>[6x]MNLTELKNTPVSELITLGENMGLENLARMRKQDIIFAILKQHAKSGEDIFGDGVLEILQDGFGFLRSADSSYLAGPDDIYVSPSQIRRFNLRTGDTISGKIRPPKEGERYFALLKVNEVNFDKPENARNKILFENLTPLHANSRLRMERGNGSTEDLTARVLDLASPIGRGQRGLIVAPPKAGKTMLLQNIAQSIAYNHPDCVLMVLLIDERPEEVTEMQRLVKGEVVASTFDEPASRHVQVAEMVIEKAKRLVEHKKDVIILLDSITRLARAYNTVVPASGKVLTGGVDANALHRPKRFFGA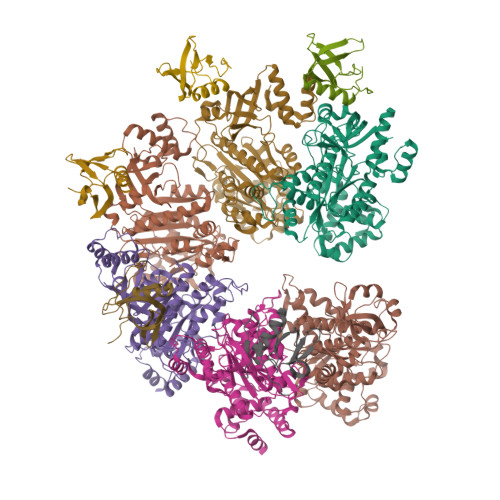ARNVEEGGSLTIIATALIDTGSKMDEVIYEEFKGTGNMELHLSRKIAEKRVFPAIDYNRSGTRKEELLTTQEELQKMWILRKIIHPMGEIDAMEFLINKLAMTKTNDDFFEMMKRS;>AMGNDTYQPINCDDYDNLELACQHHLMLTLELKDGEKLQAKASDLVSRKNVEYLVVEAAGETRELRLDKITSFSHPEIGTVVVSES[5x]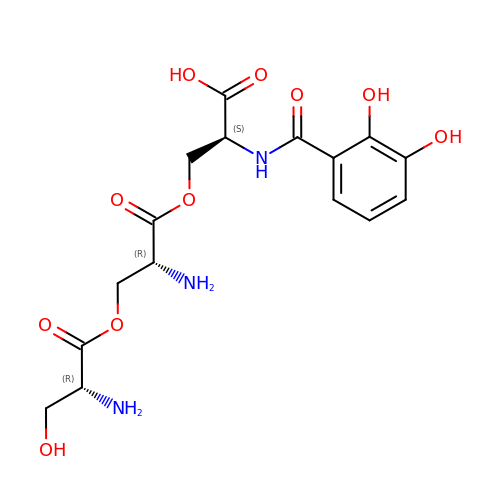O-[(2R)-2-amino-3-(D-seryloxy)propanoyl]-N-[(2,3-dihydroxyphenyl)carbonyl]-L-serine | C16 H21 N3 O10 | ZXSIADNPWRCRTI-BBBLOLIVSA-N> GPYLQILEQPKQRGFRFRYVCEGPSHGGLPGASSEKNKKSYPQVKICNYVGPAKVIVQLVTNGKNIHLHAHSLVGKHCEDGVCTVTAGPKDMVVGFANLGILHVTKKKVFETLEARMTEACIRGYNPGLLVHSDLAYLQAEGGGDRQ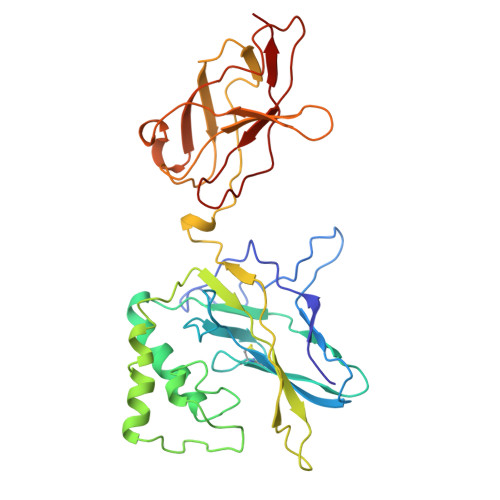LTDREKEIIRQAAVQQTKEMDLSVVRLMFTAFLPDSTGSFTRRLEPVVSDAIYDSKAPNASNLKIVRMDRTAGCVTGGEEIYLLCDKVQKDDIQIRFYEEEENGGVWEGFGDFSPTDVHRQFAIVFKTPKYKDVNITKPASVFVQLRRKSDLETSEPKPFLYYPE>QPWEAIFTKDDLAAIEPKPASANVPNTKQWIGIQAGLIKAGATDANFMKVLLGLSLEAFDRGSSEATTWDGITEGVEHRAAANAIKEANCPIHKVTYYLAKPTFAIRQSKNLPPANFAKKNVPSQYKWCAFDA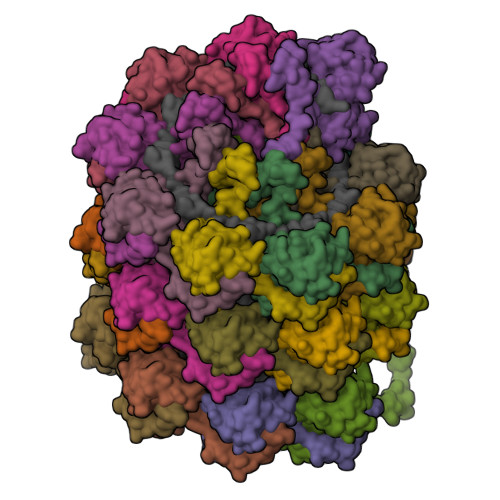FDGLYDPTCLASELPYDAPSEIDRMAYATFKTIQIKIANDQKGFNLNYNPNVTQARLPNAPLPALPEPTSD[25x]> AKLRQFYVAAQSIRWNYRPESTHLSSKPFETSFKKIVYREYEAYFQKEKPQSRTSGLLGPTLYAEVGDIMKVHFKNKAHKPLSIHAQGIKYSKFSEGASYSDHTLPMEKMDDAVAPGQEYTYEWIISEHSGPTHDDPPCLTHIYYSYVNLVEDFNSGLIGPLLICKKGTLTEDGTQKMFEKQHVLMFAVFDESKSWNQTSSLMYTVNGYVNGTMPDITVCAHDHISWHLIGMSSGPELFSIHFNGQVLEQNHHKISAITLVSATSTTANMTVSPEGRWTIASLIPRHFQAGMQAYIDIKNCAKKTR;> SNTGNRKYYYIAAEEISWDYSKFVQSDDVDYVPEDTVYKKVVFRKYLDSTFTKLDPQGEYEEHLGILGPVIRAEVDDVIQVRFKNLASRPYSLHAHGLSYEKSSEGKTYEDDSPEWFKEDNAIQPNKTYTYVWHATTRSGPENPGSACRAWAYYSAVNPEKDIHSGLIGPLLICRKGTLDKETNMPVDMREFVLLFMVFDEKKSWYYDKKPTRSWRRASSEVKNSHEFHAINGMIYNLPGLRMYEQEWVRLHLLNLGGSRDIHVVHFHGQTLLENGTQQHQLGVWPLLPGSFKTLEMKASKPGWWLLDTEVGEIQRAGMQTPFL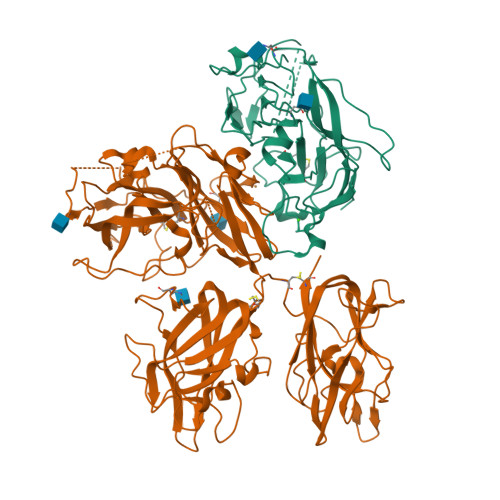IVDRECKMPMGLSTGLIADSQIQASEFWGYWEPKLARLNNGGSYNAWIAEKLSTEFNPEPWIQVDMQKEVLLTGIQTQGAKHYLKPYYTTEFCVAYSLDRKNWRIFKGNSTRNVMYFGGNSDASTIKENQIDPPVVARYIRISPTGSYNKPALRLELQGCEVNGCSTPLGMESGKIENKQITASSFKKSWWGNYWEPFLARLNAQGRVNAWQAKANNNNQWLQIDLLKIKKITAIVTQGCKSLSSEMYVKSYTIHYSDQGTDWKPYREKSSMVDKIFEGNNNVRGHVKNFFNPPIISRFIRIIPKTWNQSIALRLELFGCDMY> VDC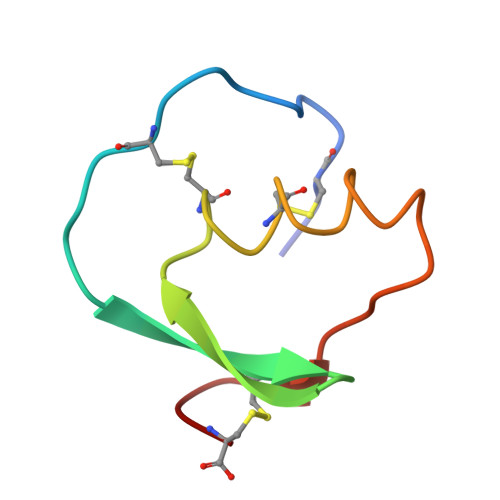SEYPKPACTFEYRPLCGSDNKTYGNKCNFCNAVVESNGTLTLSHFGKC The PHDs are Fe(II)/2‐oxoglutarate (2OG) oxygenases that catalyse hydroxylation of prolyl‐residues in the oxygen degradation domains (ODDs) of HIFα. The oxygen‐dependent prolyl hydroxylation of HIFα isoforms signals for their degradation via the ubiquitin‐proteasome system. Inhibition of the hypoxia inducible factor (HIF) prolyl hydroxylases (human PHD 1–3), with consequent increases in HIF levels, is being pursued for treatment of anaemia (via increasing erythropoietin) and has potential for treatment of other ischemia‐related diseases. We report structure–activity relationship and crystallographic studies on a promising class of 4‐hydroxypyrimidine‐containing PHD inhibitors.

To explore diversification of binding in the hydrophobic pocket at the PHD active site entrance, we selected the 4‐hydroxy‐2‐(1H‐pyrazol‐1‐yl)pyrimidine scaffold because we predicted its C‐5 amide group would bind to the PHDs analogously to the C‐3 group of the spiro[4.5]decanone series. An X‐ray crystal structure of a truncated domain of PHD2 (tPHD2) with MnII (substituting for FeII) and complexed with 8 was obtained. The overall fold is similar to previously reported PHD‐inhibitor complex structures (backbone root mean square deviation with a structure of tPHD with 18: 0.7564) (S2‐3).7 The structure reveals a binding mode for 8 involving chelation of the active site metal via nitrogen atoms of the pyrazolo and a pyrimidyl rings which adopt a coplanar conformation. The pyrazole ring of 8 occupies the entrance of the active site pocket that is occupied by the CH2CO2H group of 2OG during catalysis. Instead of interacting with an inhibitor carboxylate, the guanidino group of Arg‐383 is positioned to interact with a formate ion, likely derived from the crystallization buffer. The terminal phenyl ring of 8 forms an edge‐face π‐stacking interaction with Phe‐391 and interacts with the Arg‐396 side chain. Recently, we reported SAR studies on spiro[4.5]decanone containing PHD inhibitors, leading to the identification of a hydrophobic pocket close to the Fe(II) binding site of the target enzymes. The side chains of Trp‐258, Trp‐389 and Phe‐391 in PHD2 are positioned to make hydrophobic and π‐stacking interactions with the biphenyl substituent of spiro[4.5]decanone derivatives. Targeting the hydrophobic pocket at the entrance to the active site of the PHDs enabled identification of 4‐hydroxy‐2‐(1H‐pyrazol‐1‐yl) pyrimidines selective for the PHDs over structurally related 2OG oxygenases. Modulation of inhibitors elements binding in this region will likely be useful for further optimizing 4‐hydroxy‐2‐(1H‐pyrazol‐1‐yl)pyrimidines potency, and for improving the cellular activity of the compounds reported here.

>GSHMASPNGQTKPLPALKLALEYIVPCMNKHGICVVDDFLGKETGQQIGDEVRALHDTGKFTDGQLVSQKSDSSKDIRGDKITWIEGKEPGCETIGLLMSSMDDLIRHCNGKLGSYKINGRTKAMVACYPGNGTGYVRHVDNPNGDGRCVTCIYYLNKDWDAKVSGGILRIFPEGKAQFADIEPKFDRLLFFWSDRRNPHEVQPAYATRYAITVWYFDADERARAKVKYLTGE[2x]>MATLAFILYKYFPFGGLQRDFMRIALECQRRGHDIRVYTL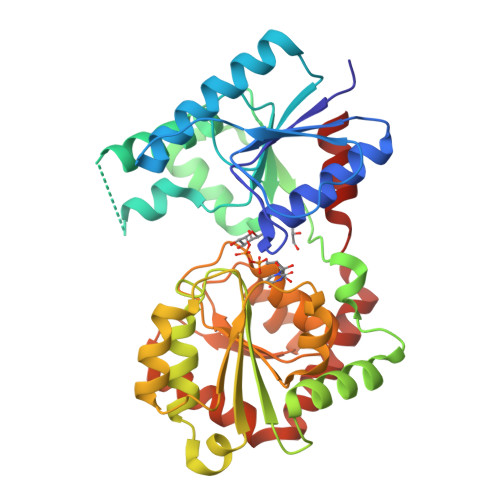IWEGDVPDGFEVLVAPVRSIFNHRRNEKFTAWVRADLDRRPVQRVIGFNKMPGLDVYYAADACFEEKAQTLRNPLYRQWGRYRHFAGYERAVFDPASKTEILMISEVQQPLFVKHYGTQAERFHLLPPGISQDRRAPANAADVRAEFRREFGLEEDDLLLVQIGSGFKTKGLDRSLKALSALPKALRRRTRLIAIGQDDPKPFLLQIAALGLNDQVQILKGRSDIPRFLLGADLLIHPAYNENTGTVLLEALVSGLPVLVTDVCGYAHYIAEADAGRVLPSPFEQDSLNRLLAEMLEDAPARAAWSRNGLAYADHADLYSMPQRAADLILG[2x]> GSSGSSGMKNIESLFDYSAGQFEF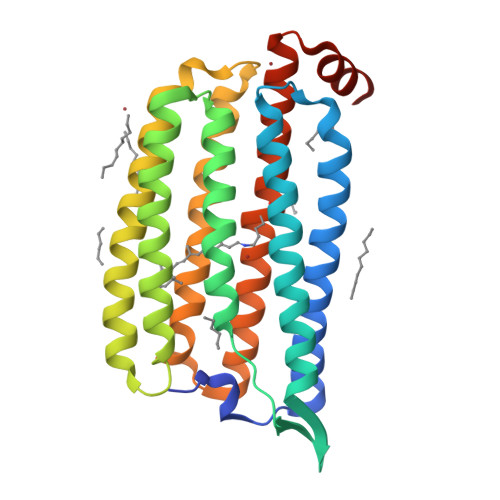IDHLLTMGVGVHFAALIFFLVVSQFVAPKYRIATALSCIVMVSAGLILNSQAVMWTDAYAYVDGSYQLQDLTFSNGYRYVNWMATIPCLLLQLLIVLNLKGKELFSTATWLILAAWGMIITGYVGQLYEVDDIAQLMIWGAVSTAFFVVMNWIVGTKIFKNRATMLGGTDSTITKVFWLMMFAWTLYPIAYLVPAFMNNADGVVLRQLLFTIADISSKVIYGLMITYIAIQQSAAAGYVPAQQALGRIGMDSKAA> 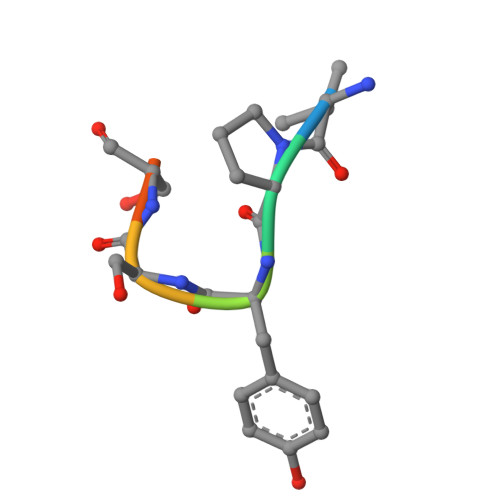VPYSSAQ>MFTLAEVASLNDIQPTYRILKPWWDVFMDYLAVVMLMVAIFAGTMQLTKDQVVCLPVLPSPVNSKAHTPPGNAEVTTNIPKMEAATNQDQDGRTTNDISFGTSAVTPDIPLRATYPRTDFALPNQEAKKEKKDPTGRKTNLDFQQYVFINQMCYHLALPWYSKYFPYLALIHTIILMVSSNFWFKYPKTCSKVEHFVSILGKCFESPWTTKALSETACEDSEE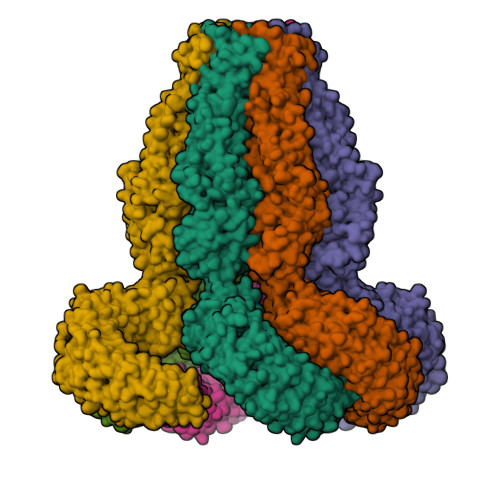NKQRITGAQTLPKHVSTSSDEGSPSASTPMINKTGFKFSAEKPVIEVPSMTILDKKDGEQAKALFEKVRKFRAHVEDSDLIYKLYVVQTVIKTAKFIFILCYTANFVNAISFEHVCKPKVEHLIGYEVFECTHNMAYMLKKLLISYISIICVYGFICLYTLFWLFRIPLKEYSFEKVREESSFSDIPDVKNDFAFLLHMVDQYDQLYSKRFGVFLSEVSENKLREISLNHEWTFEKLRQHISRNAQDKQELHLFMLSGVPDAVFDLTDLDVLKLELIPEAKIPAKISQMTNLQELHLCHCPAKVEQTAFSFLRDHLRCLHVKFTDVAEIPAWVYLLKNLRELYLIGNLNSENNKMIGLESLRELRHLKILHVKSNLTKVPSNITDVAPHLTKLVIHNDGTKLLVLNSLKKMMNVAELELQNCELERIPHAIFSLSNLQELDLKSNNIRTIEEIISFQHLKRLTCLKLWHNKIVTIPPSITHVKNLESLYFSNNKLESLPVAVFSLQKLRCLDVSYNNISMIPIEIGLLQNLQHLHITGNKVDILPKQLFKCIKLRTLNLGQNCITSLPEKVGQLSQLTQLELKGNCFDRLPAQLGQCRMLKKSGLVVEDHLFDTLPLEVKEALNQDINIPFANGIGTENLYFQ[6x]> AGSLKPAALYEEALSLVKDGDVACRSLRTELLECYSDQDFLAKLHCVRQAFQVLLLDETHRMFFMETGKQMISGLLVKANKSPKAFLESYEDMLQYTQREETWPVSKMELEGRGVVCMNFFDIVLDFILMDAFEDLESPPSSVVAVLRNRWLSDSFKETALATACWSVLKAKRRLLMVPDGFIAHFYVISEHVSPVLAFGFLGPHQHLSEVCTIFKQQIVQYLKDMF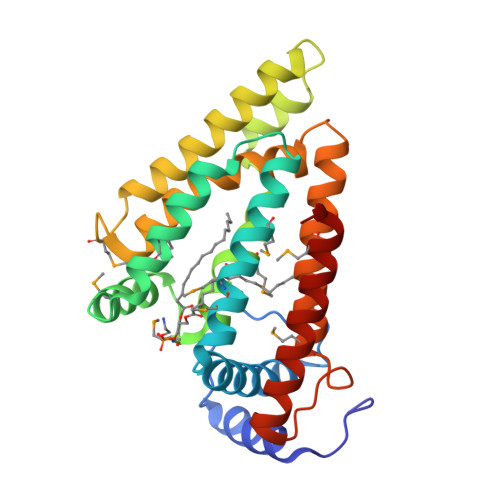DHDKVRFTSVPSLAEDILRLSHRRADILMGYLGIE>DRMKIGASLADVDPMQLDSSVRFDSVGGLSNHIAALKEMVVFPLLYPEVFEKFKIQPPRGCLFYGPPGTGKTLVARALANECSQGDKRVAFFMRKGADCLSKWVGESERQLRLLFDQAYQMRPSIIFFDQIDGLAPVRSSRQDQIHSSIVSTLLALMDGLDSRGEIVVIGATNRLDSIDPALRRPGRFDREFLFSLPDKEARKEILKIHTRDWNPKPLDTFLEELAENCVGYCGADIKSICAEAALCALRRRYPQIYTTSEKLQLDLSSINISAKDFEVAMQKMIPASQRAVTSPGQALSTVVKPLLQNTVDKILEALQRVFPHAEFRTNKTLDSDISCPLLESDLAYSDDDVPSVYENGLSQKSSHKAKDNFNFLHLNRNACYQPMSFRPRILIVGEPGFGQGSHLAPAVIHALEKFTVYTLDIPVLFGVSTTSPEETCAQVIREAKRTAPSIVYVPHIHVWWEIVGPTLKATFTTLLQNIPSFAPVLLLATSDKPHSALPEEVQELFIRDYGEIFNVQLPDKEERTKFFEDLILKQAAKPPISKKKAVLQALEVLPVAPPPEPRSLTAEEVKRLEEQEEYAPSYYHVMPKQNSTLVGDKRSDPEQNEKLKTPSTPVACSTPAQLKRKIRKKSNWYLGTIKKRRKISQAKDDSQNAIDHKIESDTEETQDTSVDHNETGNTGESSVEENEKQQNASESKLELRNNSNTCNIENELEDSRKTTACTELRDKIACNGDASSSQIIHISDENEGKEMCVLRMTQPTPSLVVDHERLKNLLKTVVKKSQNYNIFQLENLYAVISQCIYRHRKDHDKTSLIQKMEQEVENFSCSR[6x]

ATAD2 is a non-canonical ATP-dependent histone chaperone and a major cancer target. From a structural standpoint, ATAD2 exhibits a conserved multidomain architecture comprising an N-terminal acidic domain, two AAA+ ATPase domains, a bromodomain, C-terminal domain, and an exceptionally long C-terminal linker (CTL) that bridges the bromo- and C-terminal domain. Unlike most other histone chaperones that do not require ATP for activity, ATAD2 stands out due to the presence of an ATP-dependent AAA+ ATPase domain. The AAA+ domain adopts a conserved structural fold found in the AAA+ ATPase superfamily, with each monomer consisting of a large α/β nucleotide binding domain (NBD) and a small α -helical bundle domain (HBD).

However, when a specific mutation (E532Q) which specifically blocks ATP-hydrolysis was introduced into the Walker B motif, ATAD2 formed stable hexamers with homogeneous particle distributions. In the hexameric structure of ATAD2, the six subunits were arranged in a right-handed spiral with a rise of ~2 Å and a rotation of ~60 ° around the helical axis. This resulted in a “seam” between the top (herein referred to as “subunit P1”) and bottom (herein referred to as “subunit P6”) subunits with an offset of ~12 Å. Five binding pockets of AAA1 were occupied by ATP, while the binding pocket of P6 at the spiral seam (P1/P6 interface) was occupied by ADP. When comparing individual ATAD2 subunits we also discovered a conserved N-terminal linker domain (aa406-423, referred to as “LD” hereafter). This structural element was only visible in the ADP-bound subunit, P6, and was sandwiched between the two subunits at the spiral seam (subunits P1 and P6). In the ATAD2 structure, a salt bridge is formed between D415 of the N-terminal LD in P6 and R540 of pore loop 2 in P1, potentially stabilizing the P6 N-terminal LD-P1 interaction and hexamerization of ATAD2. Third, while translocating AAA+ ATPases usually have 5 to 6 subunits engaged with the substrate in the active state, only 3 ATAD2 subunits (P2-4) engaged with substrate, suggesting a “weak grip”. Second, we observe the N-terminal LD of the P6 subunit wedged between the seam subunits, where it effectively glues the P1 and P6 subunits in place, thus limiting subunit translocation and symmetry breaking. Third, only three ATAD2 pore loops maintain a weak grip on a short length of substrate in the central substrate, hinting at a non-productive or weakly-productive state if ATAD2 were to pull on substrates. Together, these lines of evidence imply that the N-terminal LD acts as a brake that maintains ATAD2 in an autoinhibited state thus preventing premature ATPase activation.>ENSGGNAFVPAGNQQEAHWTINLKDADIREFIDQISEITGETFVVDPRVKGQVSVVSKAQLSLSEVYQLFLSVMSTHGFTVVAQGDQARIVPNAEAKTEAGGGQSAPDRLETRVIQVQQSPVSELIPLIRPL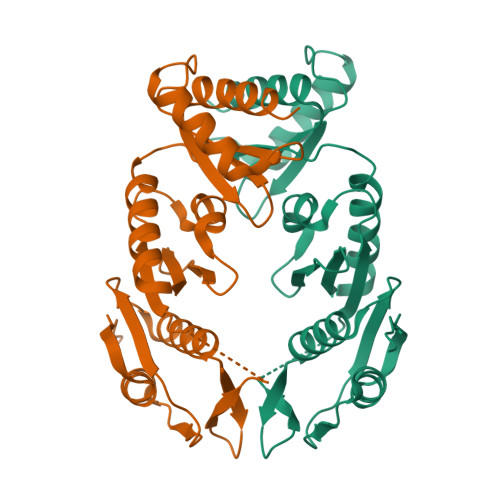VPQYGHLAAVPSANALIISDRSANIARIEDVIRQLDQKGSHDYSVINLRYGWVMDAAEVLNNAMSRGQAKGAAGAQVIADARTNRLIILGPPQARAKLVQLAQSLDTPT[2x]>MKGLAMLGIGRIGWIEKKIPECGPLDALVRPLALAPCTSDTHTVWAGAIGDRHDMILGHEAVGQIVKVGSLVKRLKVGDKVIVPAITPDWGEEESQRGYPMHSGGMLGGWKFSNFKDGVFSEVFHVNEADANLALLPRDIKPEDAVMLSDMVTTGFHGAELANIKLGDTVCVIGIGPVGLMSVAGANHLGAGRIFAVGSRKHCCDIALEYGATDIINYKNGDIVEQILKATDGKGVDKVVIAGGDVHTFAQAVKMIKPGSDIGNVNYLGEGDNIDIPRSEWGVGMGHK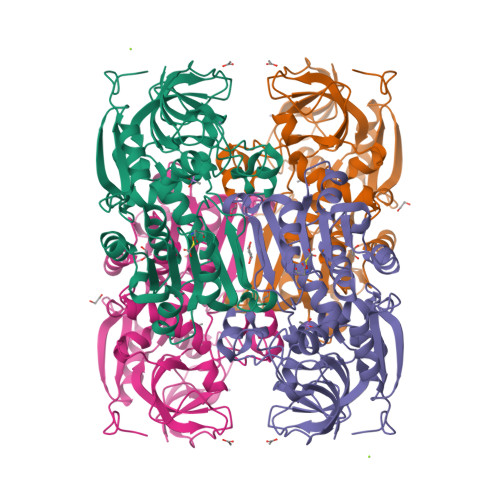HIHGGLTPGGRVRMEKLASLISTGKLDTSKLITHRFEGLEKVEDALMLMKNKPADLIKPVVRIHYDDEDTLH[2x]Herein, we describe the use of GE to optimize a fragment‐derived inhibitor of Mycobacterium tuberculosis pantothenate synthetase, an attractive target for developing new drugs against tuberculosis. Pantothenate synthetase catalyzes the ATP‐dependent formation of an amide bond between pantoate and β‐alanine. The work presented here demonstrates the use of GE analysis to critically and thoroughly examine the binding distribution of a lead compound and illustrates the practicality of applying GE analysis to modify parts of a molecule that are not making efficient contributions to binding. In this case, it led to the generation of a relatively potent and bactericidal inhibitor of M. tuberculosis pantothenate synthetase.

Based on these observations, the initial optimization strategy was focused on replacement of the methyl pyridine and the benzofuran groups rather than the acyl sulfonamide linker in both compounds 5 and 8. Compounds were designed with the objective of optimizing interactions at the P1 or P2 sites of panthothenate synthetase. Consequently, 1‐ethyl‐3‐(3‐dimethylaminopropyl)‐carbodiimide (EDCI)‐mediated coupling reactions were employed to generate a series of indole acyl sulfonamide compounds (10–19; the syntheses are described in the Supporting Information). In order to establish this, the structures of the four most potent inhibitors (10–13) bound to the enzyme were solved using protein X‐ray crystallography. The X‐ray crystal structures of 10–13 bound to pantothenate synthetase show binding at the active site, with a conserved binding mode for the indole sulfonamide fragment core. Less obviously, the substituted groups on all four compounds were seen to bind in the P1 pocket of the enzyme. The P1 pocket binds the alkyl groups of the pantoate substrate and is primarily lipophilic, surrounded by the hydrophobic residues Pro 38, Met 40, Val 143, Leu 146 and Phe 157. In contrast, the P2 site binds the phosphates of ATP and is relatively hydrophilic. As can be seen in Figure 2, the binding orientations of the added groups are all similar, and no new hydrogen bonds are formed. In addition to binding assays and X‐ray crystallography studies, an inhibition study was carried out that demonstrated that compound 11 inhibits pantothenate synthetase with an IC50 value of 5.7 μm.

>MAIPAFHPGELNVYSAPGDVADVSRALRLTGRRVMLVPTMGALHEGHLALVRAAKRVPGSVVVVSIFVNPMQFGAGGDLDAYPRTPDDDLAQLRAEGVEIAFTPTTAAMYPDGLRTTVQPGPLAAELEGGPRPTHFAGVLTVVLKLLQIVRPDRVFFGEKDYQQLVLIRQLVADFNLDVAVVGVPTVREADGLAMSSRNRYLDPAQRAAAVALSAALTAAAHAATAGAQAALDAARAVLDAAPGVAVDYLELRDIGLGPMPLNGSGRLLVAARLGTTRLLDNIAIEIGTFAGTDRPDGYR[2x]> GKITFYEDRGFQG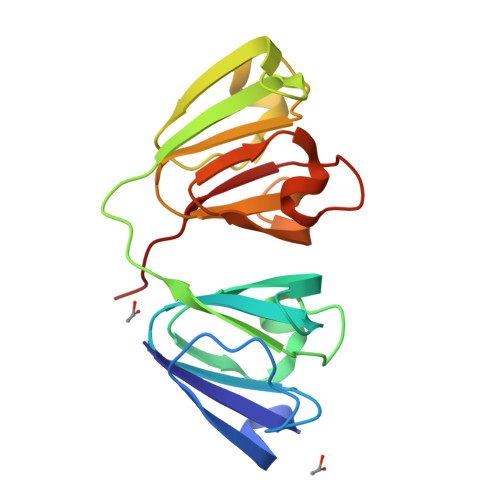RHYECSTDHSNLQPYFSRCNSVRVDSGCWMLYEQPNFTGCQYFLRRGDYPDYQQWMGFSDSVRSCRLIPHSSSHRIRIYEREDYRGQMVEITDDCPHLQDRFHFSDFHSFHVMEGYWVLYEMPNYRGRQYLLRPGEYRRYHDWGAMNARVGSLRRIMDFY> GAHMAGGRSWCLRRVGMSAGWLLLEDGCEVTVGRGFGVTYQLVSKICPLMISRNHCVLKQNPEGQWTIMDNKSLNGVWLNRA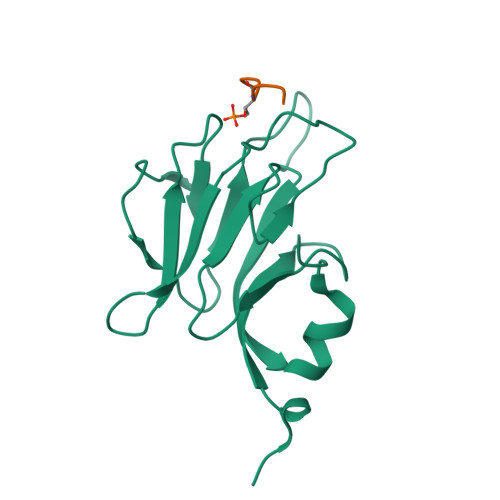RLEPLRVYSIHQGDYIQLGVPLENKENAEYEYEVTEEDWETIYPCLSPKNDQMIEK;> ELKTERY>MYRSHFIADVTPEYDGKEVIWAGWVHLLRDLGGKKFIILRDKTGLGQVVVDKNSSAFGISQELTQESVIQVRGIVKADKRAPRGIELHAEEITLLSKAKAPLPLDVSGKVKADIDTRLRERVLDLRRQEMQAVIKIQSLALKAFRETLYKEGFIEIFTPKIIASATEGGAQLFPVIYFGK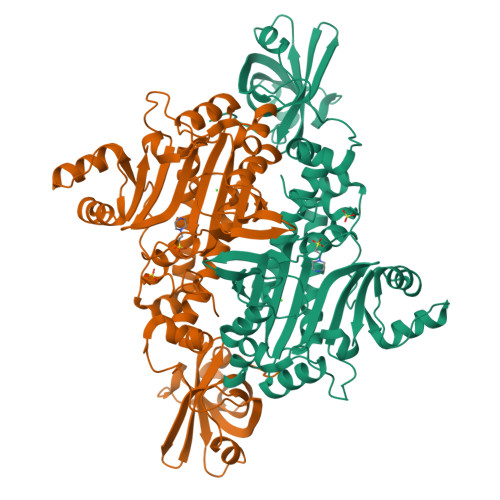EAFLAQSPQLYKELMAGVVERVFEVAPAWRAEESDTPFHLAEFISMDVEMAFADYNDVMQLLEKILHNIVKTIKEEGKEELKILNYEPPEVKIPIKRLKYTEAIEILRSKGYNIKFGDDIGTPELRILNEELKEDLYFIVDWPSDARPFYTKSKSENPELSESFDLIYKFLEIVSGSTRNHKREVLEEALKKKGLKPESFEFFLKWFDYGMPPHAGFGMGLARLMVMLTGIQSVKEIVPFPRDKKRLTP[2x]>[12x]HYASKKSAAESMLD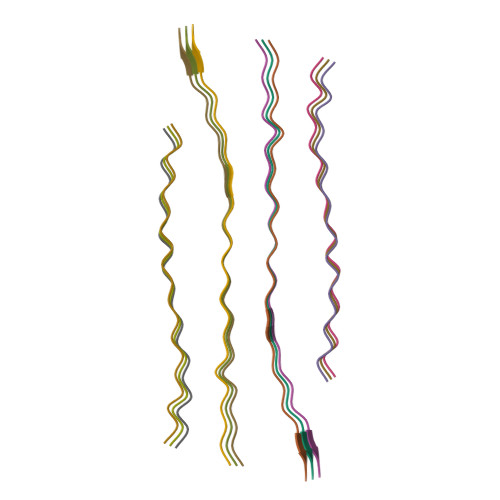IALLMANASQLKAVVE>SEAQQFTEFWTPGKPNPSICKSPLLVSTPLGLPRCLQASNVVKRLQKLEDIASLNDGNRAAATPGYQASVDYVKQTLQKAGYKVSVQPFPFTAYYPKGPGSLSATVPQPVTYEWEKDFTYLSQTEAGDVTAKVVPVDLSLGAGNTSTSGCEAEDFANFPAGSIALIQRGTCNFEQKAENAAAAGAAGVIIFNQGNTDDRKGLENVTVGESYEGGIPVIFATYDNGVAWSQTPDLQLHLVVDVVRKKTETYNVVAETRRGNPNNVVMVGAHLDSVFEGPGINDNGSGSAAQLEMAVLLAKALPVNKVRFAWWGAEEAGLVGSTHYVQNLAPEEKKKIKAYLNFDMIGSPNFGNFIYDGDGSDFGLQGPPGSAAIERLFEAYFRLRGQQSEGTEIDFRSDYAEFFNSGIAFGGLFTGAEGLKTEEQAQKYGGTAGKAYDECYHSKCDGIANINQDALEIHSDAMAFVTSWLSLSTKVVDDEIAAAGQKAQSRSLQMQKSASQIERWGHDFIK[2x]

Here we investigated the aminopeptidase, P. aeruginosa aminopeptidase (PaAP) from P. aeruginosa, which is highly abundant in the biofilm matrix. PaAP is associated with biofilm development and contributes to nutrient recycling. We confirmed that post-translational processing was required for activation and PaAP is a promiscuous aminopeptidase acting on unstructured regions of peptides and proteins. PaAP contains an M28 Zn peptidase domain (residues 44–116 and 274–510) and a PA domain (residues 117–273).

We solved the structure of PaAP in multiple forms, which revealed an interesting self-inhibitory mechanism involving the PA domain and the propeptide C-terminus. The structure of full-length PaAP was solved to 1.4 Å, and traceable between residues 44 to 536 with a 16 amino acid region (QKAQSRSLQMQKSASQ) near the C-terminus, which lacked density. However, the final ten amino acids (IERWGHDFIK) of the C-terminus could be unambiguously traced. Interestingly, in the structure of PaAP, following a short region of disorder, the C-terminus (IERWGHDFIK, residues 527–536) binds in the cleft between the PA and peptidase domain. This short propeptide region is structured, folding with a hairpin turn. A short (1-2aa) β-sheet of four strands runs through the C-terminus and PA domain. The carboxy terminus interacts with the side chain of R194. Side chains of H532 and D533 of the β-hairpin coordinate a water molecule and are positioned directly above the active site pocket. The location of the C-terminus appears to block access to the active site residues. Full-length PaAP had low activity, consistent with previous reports that PaAP is secreted as a 58 kDa propeptide (Pro-PaAP), which requires C-terminal processing to yield an active enzyme.> MYFSEQNKMIRKLARDFAEKELT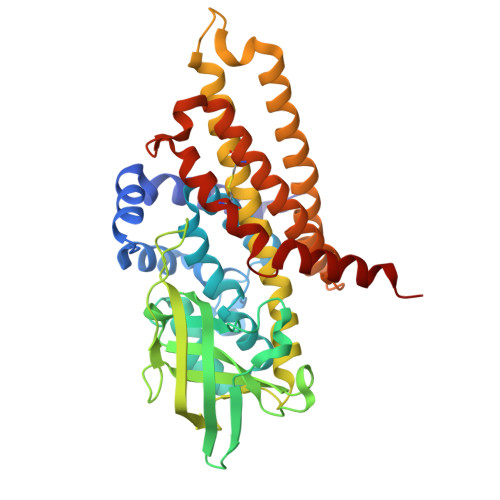TEILDEVEESGEFPQEILDKMAKFGFFGIKIPKSLGGSGGDHMSYVICMEEFARVSGVASVYLSSPNSLAGGPLLLSGTEEQIEKYLKPIITGKKKLAFALTEPGAGSDAGGMSTTAVDMGDYYLLNGRKTFITMAPLCDDAVIYAKTDMSKGTRGISAFIVDLKSEGVSMGKNEHKMGLIGCATSDIIMEDVKVPKENRLGEVNKGFSNAMKTLDVGRLGVASQSIGVAQGALDEAIKYAKERKQFGKRIADFQAIAFMIADMATKLEAAKLLVYNAASLMDNKKNATKEASMAKFYASEICNEICAKAVQIHGGYGYIKEYKVERMYRDCRVFTIYEGTSQVQQMVISGMLLKK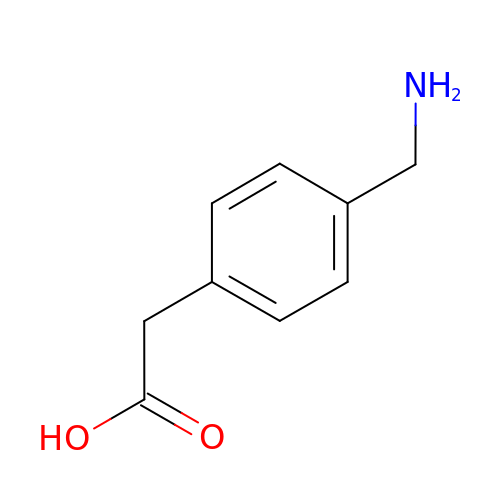2-[4-(aminomethyl)phenyl]ethanoic acid | C9 H11 N O2 | HAAUVXXFRQXTTQ-UHFFFAOYSA-N>[8x]SNAMAGTLDLDKGCTVEELLRGCIEAFDDSGKVRDPQLVRMFLMMHPWYIPSSQLAAKLLHIYQQSRKDNSNSLQVKTCHLVRYWISAFPAEFDLNPELAEQIKELKALLDQEGNRRHSSLIDIDSVPTYKWKRQVTQRNPVGQKKRKMSLLFDHLEPMELAEHLTYLEYRSFCKILFQDYHSFVTHGCTVDNPVLERFISLFNSVSQWVQLMILSKPTAPQRALVITHFVHVAEKLLQLQNFNTLMAVVGGLSHSSISRLKETHSHVSPETIKLWEGLTELVTATGNYGNYRRRLAACVGFRFPILGVHLKDLVALQLALPDWLDPARTRLNGAKMKQLFSILEELAMVTSLRP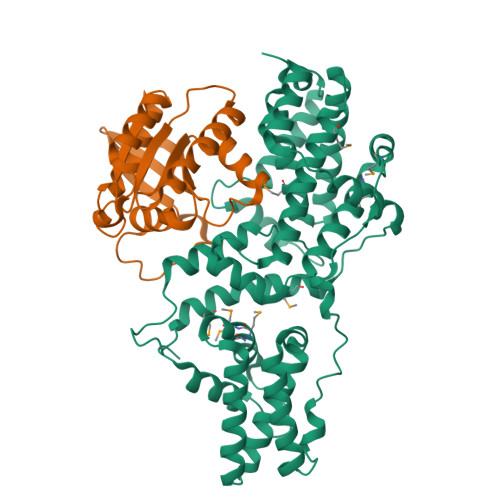PVQANPDLLSLLTVSLDQYQTEDELYQLSLQREPRSKSSPTS;>GAMREYKLVVLGSGGVGKSALTVQFVQGIFVEKYDPTIEDSYRKQVEVDAQQCMLEILDTAGTEQFTAMRDLYMKNGQGFALVYSITAQSTFNDLQDLREQILRVKDTDDVPMILVGNKCDLEDERVVGKEQGQNLARQWNNCAFLESSAKSKINVNEIFYDLVRQINR[8x]> GP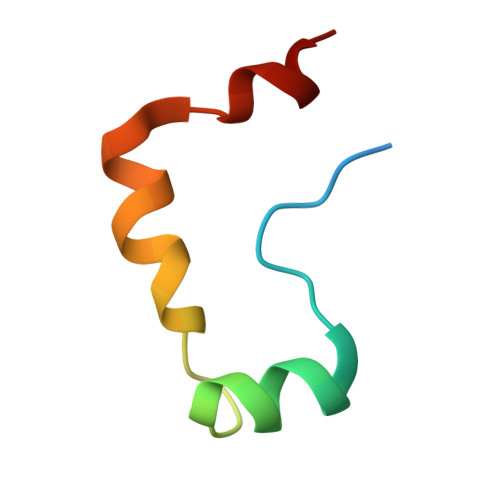DSMRFKPGVISEELQDALGVTDKSLPPFIYRMRQLGYPPGWLK> KPRGKRGWLWLLLKLAIVFAVLIAIYGVYLDQKIRSRIDGKVWQLPAAVYGRMVNLEPDMTISKNEMVKLLEATQYRQVSKMTRPGEFTVQANSIEMIRRPFDFPDSKEGQVRARLTFDGDHLATIVNMENNRQFGFFRLDPRLITMISSPNGEQRLFVPRSGFPDLLVDTLLATEDRHFYEHDGISLYSIGRAVLANLTAGRTVQGASTLTQQLVKNLFLSSERSYWRKANEAYMALIMDARYSKDRILELYMNEVYLGQSGDNEIRGFPLASLYYFGRPVEELSLDQQALLVGMVKGASIYNPWRNPKLALERRNLVLRLLQQQQIIDQELYDMLSARPLGVQPRGGVISPQPAFMQLVRQELQAKLGDKVKDLSGVKIFTTFDSVAQDAAEKAAVEGIPALKKQRKLSDLETAIVVVDRFSGEVRAMVGGSEPQFAGYNRAMQARRSIGSLAKPATYLTALSQPKIYRLNTWIADAPIALRQPNGQVWSPQNDDRRYSESGRVMLVDALTRSMNVPTVNLGMALGLPAVTETWIKLGVPKDQLHPVPAMLLGALNLTPIEVAQAFQTIASGGNRAPLSALRSVIAEDGKVLYQSFPQAERAVPAQAAYLTLWTMQQVVQRGTGRQLGAKYPNLHLAGKTGTTNNNVDTWFAGIDGSTVTITWVGRDNNQPTKLYGASGAMSIYQRYLANQTPTPLNLVPPEDIADMGVDYDGNFVCSGGMRILPVWTSDPQSLCQQSEMQQQPS;> LPPKPEERWRYIKELESRQ

PBP1b has a modular structure, composed of an N-terminal tail and a transmembrane anchor followed by the GTase and TPase catalytic domains separated by the regulatory UB2H domain. PBP1a is mainly involved in cell elongation in partnership with PBP2, whereas PBP1b exhibits a preference for cell division in agreement with its enrichment at midcell during cell constriction. In Escherichia coli, septal PG synthesis and cell constriction rely on the accumulation of FtsN at the division site. Here, we show that EFtsN binds specifically to the major PG synthase PBP1b and is sufficient to stimulate its biosynthetic glycosyltransferase (GTase) activity.

Having strong evidence of the binding of EFtsN to PBP1b, we performed co-crystallization assays between PBP1b (positions 58–804), in both the presence and the absence of moenomycin A, which helps in the crystallization of PBP1b, and purified EFtsN (Leu75–Gln93) peptide to identify the binding site of this domain on PBP1b. Crystals, which were only obtained in the presence of moenomycin A, belong to the space group P21212, similar to those of previously reported for PBP1b structures. The structure was solved to 2.4 Å resolution by molecular replacement and showed an additional electron density between the GTase and the UB2H domains. An attempt at shifting the sequence in both directions on the helix did not lead to improved Rfree or electron density. This 13-amino acid helix mostly interacts with the GTase domain and runs approximately parallel to its last α12 helix. Three hydrogen bonds are observed with PBP1b, between the side chain of Trp83 and the main-chain carbonyl of Gln384 (α11α12 loop, GTase domain), between the main-chain carbonyl of Leu89 and side-chain hydroxyl of Thr140 (α1β2 loop, UB2H domain), and between the Glu90 side chain and the Arg141 side chain (α1β2 loop, UB2H), as well as the Leu344 main chain (α9α10 loop, GTase). The GTase domain accounts for most of the interaction with EFtsN, but two residues (Thr140 and Arg141) in the α1β2 loop of the UB2H domain pointing toward the GTase domain are also involved in the binding. Furthermore, the structure reveals that the conserved residues Trp83, Tyr85, and Leu89 of EFtsN, which were shown to be important for the in vivo function of the protein, together with Ile86 and Glu90 are directly involved in the interaction with PBP1b. The binding site of EFtsN is distinct from that of LpoB, which binds the exposed surface of UB2H domain. In the structure of the PBP1b–EFtsN complex, the GTase domain is also characterized by overall poorer electron densities compared with the rest of the protein as well as, compared with the GTase domains of other structures available.> MSEESQAFQRQLTALIGYDVTDVSNVHDDELEFTRRGLVTPRMAEVASRDPKLYAMHPWVTSKPLPEYLWKKIANNCIFIVIHRSTTSQTIKVSPDDTPGAILQSFFTKMAKKKSLMDIPESQSEQDFVLRVCGRDEYLVGETPIKNFQWVRHCLKNGEEIHVVLDTPPDPALDEVRKEEWPLVDDCTGVTGYHEQLTIHGKDHESVFTVSLWDCDRKFRVKIRGIDIPVLPRNTDLTVFVEANIQHGQQVLCQRRTSPKPFTEEVLWNVWLEFSIKIKDLPKGALLNLQIYCGKAPALSSKASAESPSSESKGKVRLLYYVNLLLIDHRFLLRRGEYVLHMWQISGKGEDQGSFNADKLTSATNPDKENSMSISILLDNYCHPIALPKHQPTPDPEGDRVRAEMPNQLRKQLEAIIATDPLNPLTAEDKELLWHFRYESLKHPKAYPKLFSSVKWGQQEIVAKTYQLLARREVWDQSALDVGLTMQLLDCNFSDENVRAIAVQKLESLEDDDVLHYLLQLVQAVKFEPY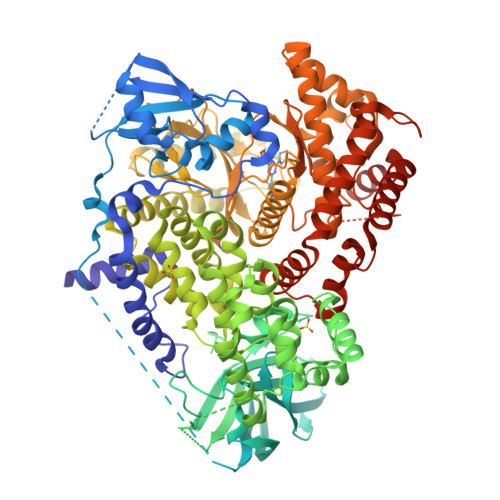HDSALARFLLKRGLRNKRIGHFLFWFLRSEIAQSRHYQQRFAVILEAYLRGCGTAMLHDFTQQVQVIEMLQKVTLDIKSLSAEKYDVSSQVISQLKQKLENLQNSQLPESFRVPYDPGLKAGALAIEKCKVMASKKKPLWLEFKCADPTALSNETIGIIFKHGDDLRQDMLILQILRIMESIWETESLDLCLLPYGCISTGDKIGMIEIVKDATTIAKIQQSTVGNTGAFKDEVLNHWLKEKSPTEEKFQAAVERFVYSCAGYCVATFVLGIGDRHNDNIMITETGNLFHIDFGHILGNYKSFLGINKERVPFVLTPDFLFVMGTSGKKTSPHFQKFQDICVKAYLALRHHTNLLIILFSMMLMTGMPQLTSKEDIEYIRDALTVGKNEEDAKKYFLDQIEVCRDKGWTVQFNWFLHLVLGIKQGEKHSAHHHHHH> QAQITGRPEWIWLALGTALMGLGTLYFLVKGMGVSDPDAKKFYAITTLVPAIAFTMYLSMLLGYGLTMVPFGGEQNPIYWARYADWLFTTP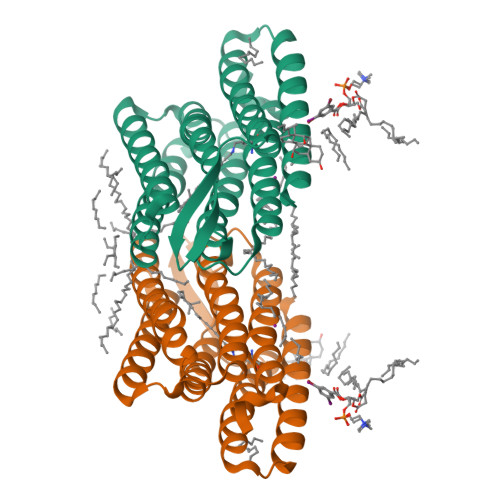LLLLDLALLVDADQGTILALVGADGIMIGTGLVGALTKVYSYRFVWWAISTAAMLYILYVLFFGFTSKAESMRPEVASTFKVLRNVTVVLWSAYPVVWLIGSEGAGIVPLNIETLLFMVLDVSAKVGFGLILLRSRAIFGEAEAPEPSAGDGAAATSD>MTPPHNYLAVIKVVGIGGGGVNAVNRMIEQGLKGVEFIAINTDAQALLMSDADVKLDVGRDSTRGLGAGADPEVGRKAAEDAKDEIEELLRGADMVFVTAGEGGGTGTGGAPVVASIARKLGALTVGVVTRPFSFEGKRRSNQAENGIAALRESCDTLIVIPNDRLLQMGDAAVSLMDAFRSADEVLLNGVQGITDLITTPGLINVDFADVKGIMSGAGTALMGIGSARGEGRSLKAAEIAINSPLLEASMEGAQGVLMSIAGGSDLGLFEINEAASLVQDAAHPDANIIFGTVIDDSLGDEVRVTVIAA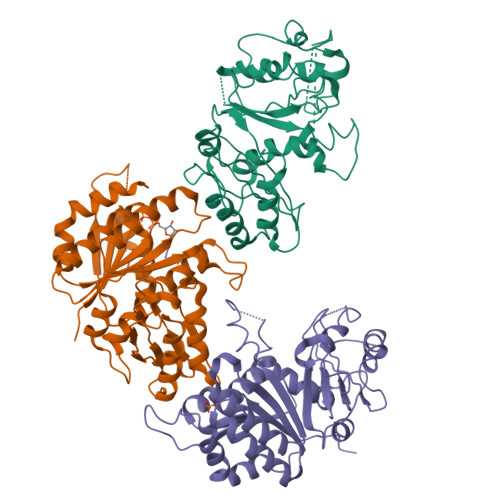GFDVSGPGRKPVMGETGGAHRIESAKAGKLTSTLFEPVDAVSVPLHTNGATLSIGGDDDDVDVPPFMRR[6x]6-(4-phenylpiperazin-1-yl)pyridine-3-carboximidamide | C16 H19 N5 | 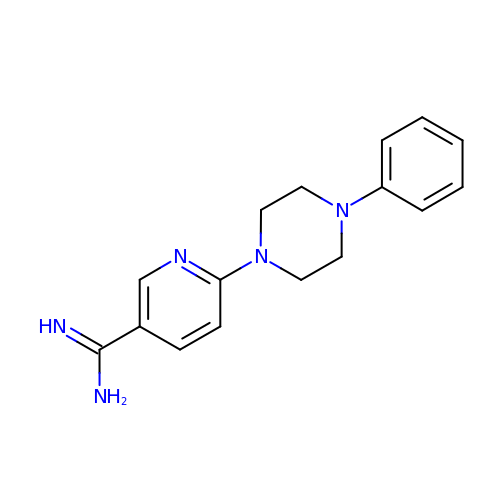UKIJUFIFFKYHSH-UHFFFAOYSA-N>MSTNKVNKERTFLAVKPDGVARGLVGEIIARYEKKGFVLVGLKQLVPTKDLAESHYAEHKERPFFGGLVSFITSGPVVAMVFEGKGVVASARLMIGVTNPLASAPGSIRGDFGVDVGRNIIHGSDSVESANREIALWFKPE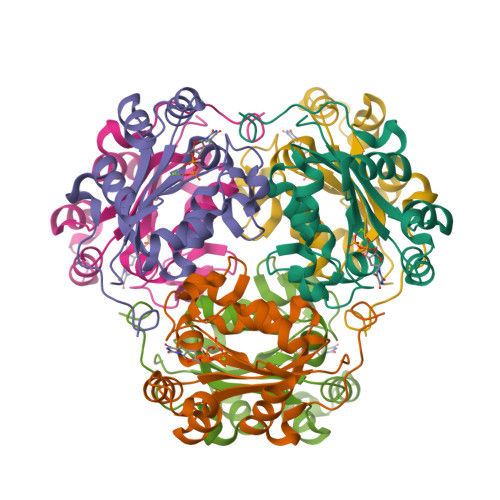ELLTEVKPNPNLYE[3x]>SHPALTQLRALRYSKEIPALDPQLLDWLLLEDSMTKRFEQQGKTVSVTMIREGFVEQNEIPEELPLLPKESRYWLREILLSADGEPWLAGRTVVPVSTLSGPELALQKLGKTPLGRYLFTSSTLTRDFIEIGRDAGLWGRRSRLRLSGKPLLLTELFLPASPL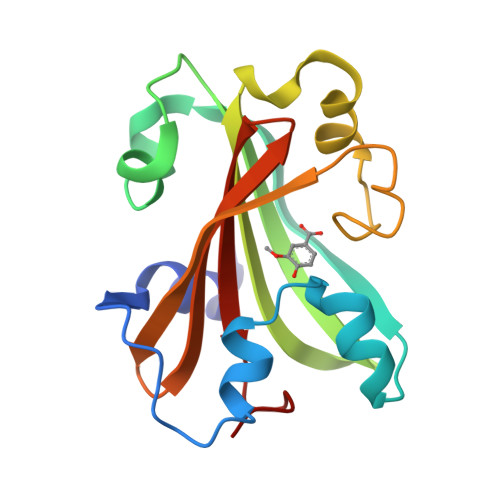Y[4x]>MASRGSHHHHHHGAYRLLNKTAVITG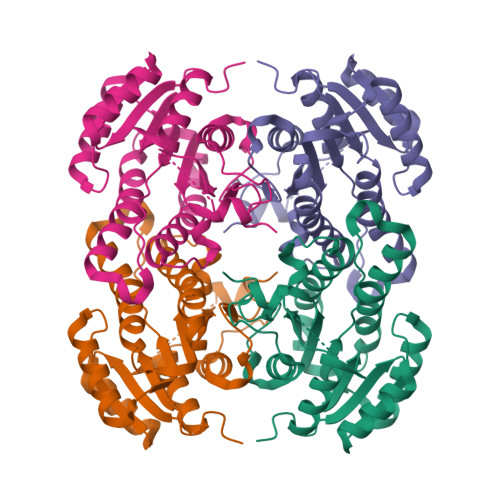GGSGIGLATAKRFVAEGAYVFIVDVSRKELEQAAAEIGRNVTAVKADVTKLEDLDRLYAIVREQRGSIDVLFANSGAIEQKTLEEITPEHYDRTFDVNVRGLIFTVQKALPLLRDGGSVILTSSVAGVLGLQAHDTYSAAKAAVRSLARTWTTELKGRSIRVNAVSPGAIDTPIIENQVSTQEEADELRAKFAAATPLGRVGRPEELAAAVLFLASDDSSYVAGIELFVDGGLTQV[8x]> RAFWHTPRLP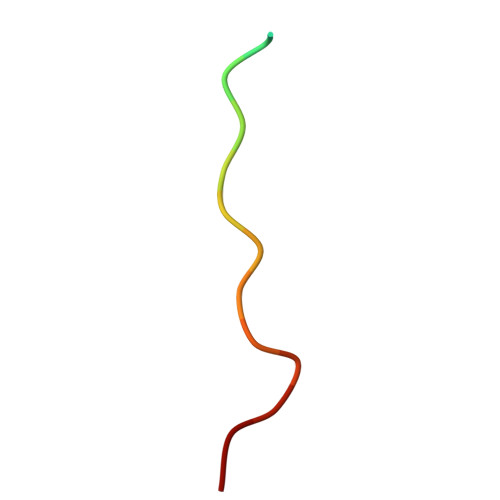TLPKRVP>MATTSNQNVEFVRTGYGKN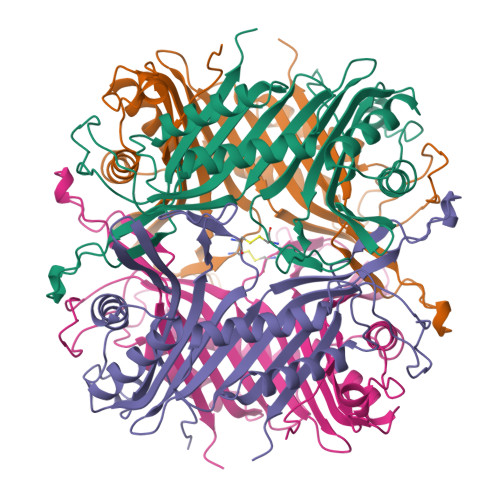MVKVLHIRREGNHHHIIELIANVQLTLKTRKDYLTGDNSDIIPTDTVKNTVHALAKLKGIKSIESFALDICEHFLTAFNHVTRVKVNIDEVPWKRLEKNGVEHNHAFIHCPEALRFCEAEQYLSKTPVVHSGLKDMKVLKTTQTGFEGFLRDRFTTLTDAKDRFFCTSVYARWRYNTINVAFDAAWKAVKDTVIQKFAGPYDRGEYSPSVQKTLYDTQLLVLDRIPEVEEIEIIMPNQHYFVIDMTKIGLSNKDEVYLPLDNPSGNITGTVCRKPRARM[8x]(2~{R})-2-[5-[3-chloranyl-2-methyl-4-[2-(4-methylpiperazin-1-yl)ethoxy]phenyl]-6-(3-chlorophenyl)thieno[2,3-d]pyrimidin-4-yl]oxy-3-(2-methoxyphenyl)propanoic 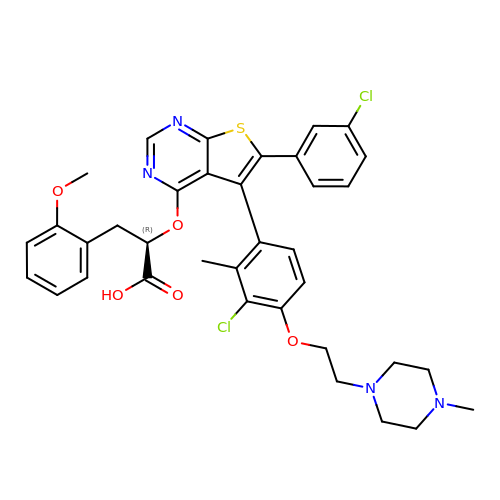acid | C36 H36 Cl2 N4 O5 S | ZDIFLDSDDULOSG-GDLZYMKVSA-N> MELTPREKDKLLLFTAALVAERRLARGLKLNYPESVALISAFIMEGARDGKSVASLMEEGRHVLTREQVMEGVPEMIPDIQVEATFPDGSKLVTVHNPII;> MIPGEYHVKPGQIALNTGRATCRVVV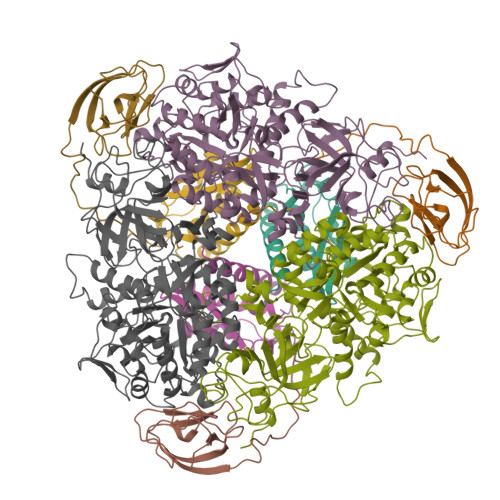ENHGDRPIQVGSHYHFAEVNPALKFDRQQAAGYRLNIPAGTAVRFEPGQKREVELVAFAGHRAVFGFRGEVMGPL;> SNISRQAYADMFGPTVGDKVRLADTELWIEVEDDLTTYGEEVKFGGGKVIRDGMGQGQMLAADCVDLVLTNALIVDHWGIVKADIGVKDGRIFAIGKAGNPDIQPNVTIPIGAATEVIAAEGKIVTAGGIDTHIHWICPQQAEEALVSGVTTMVGGGTGPAAGTHATTCTPGPWYISRMLQAADSLPVNIGLLGKGNVSQPDALREQVAAGVIGLEIHEDWGATPAAIDCALTVADEMDIQVALHSDTLNESGFVEDTLAAIGGRTIHTFHTEGAGGGHAPDIITACAHPNILPSSTNPTLPYTLNTIDEHLDMLMVCHHLDPDIAEDVAFAESRIRRETIAAEDVLHDLGAFSLTSSDSQAMGRVGEVILRTWQVAHRMKVQRGALAEETGDNDNFRVKRYIAKYTINPALTHGIAHEVGSIEVGKLADLVVWSPAFFGVKPATVIKGGMIAIAPMGDINASIPTPQPVHYRPMFGALGSARHHCRLTFLSQAAAANGVAERLNLRSAIAVVKGCRTVQKADMVHNSLQPNITVDAQTYEVRVDGELITSEPADVLPMAQRYFLF>LHETSKEPDVSLGSTWLSDFPQAWAETGGMGLAVRQAPLIIPLKATSTPVSIKQYPMSQEARLGIKPHIQRLLDQGILVPCQSPWNTPLLPVKKPGTNDYRPVQDLREVNKRVEDIHPTVPNPYNLLSGLPPSHQWYTVLDLKDAFFCLRLHPTSQPLFAFEWRDPEMGISGQLTWTRLPQGFKNSPTLFDEALHRDLADFRIQHPDLILLQYVDDLLLAATSELDCQQGTRALLQTLGNLGYRASAKKAQ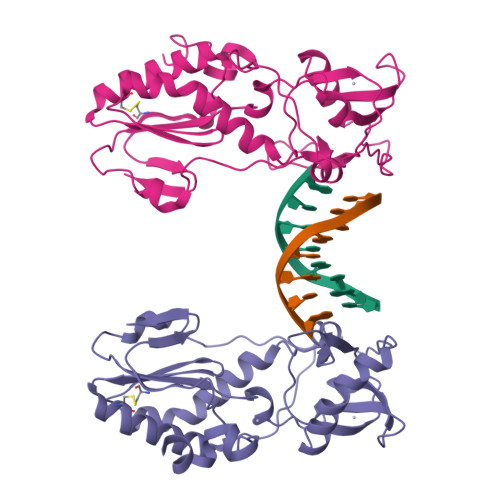ICQKQVKYLGYLLK[2x]>GPGGAASATPDVDPDDRVYIVRAQRPTYVHWAIRKVAPDGSAKQISLSRSGIQALVALEPPEGEPYLEILPSHWTLAELQLGNKWEYSATNNCTHFVSSITGE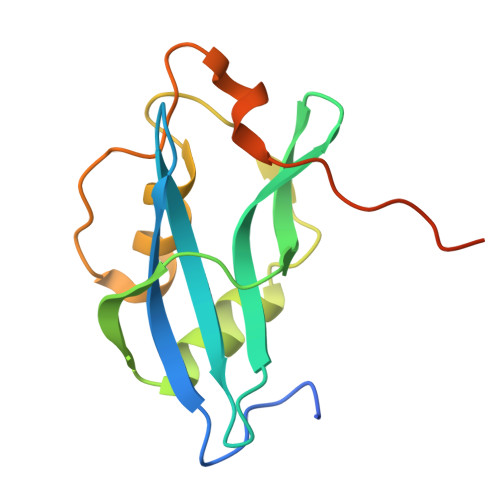SLPNTGFSLALGIGALTAIAASAAVAVKALPGIRRQ[3x]The p21-activated kinase (PAK) family comprises six sterile-20 group serine/threonine kinases. In contrast, the type II PAKs bind the Rho-family small GTPases CDC42, RAC1 and RhoV, but are not directly activated by this interaction. The type II PAKs are important for signaling cascades that regulate cell survival, neurite outgrowth and formation of filipodia. We discovered that PAK6 is inhibited by its pseudosubstrate sequence.

The small molecule PF-3758309 was designed as a PAK4-specific inhibitor, but displays in vitro activity against each of the type II PAKs and also PAK1. Though effective in mouse models of cancer, it failed in human clinical trials. We go on to determine crystal structures of PAK6 kinase domain in complex with two ATP-competitive small molecule inhibitors, PF-3758309 and sunitinib. We obtained crystals of PAK6 kinase domain in complex with either PF-3758309 or sunitinib by co-crystallization. These co-crystals diffracted X-rays to Bragg spacings of 1.40 Å and 1.95 Å respectively for the PF-3758309 and sunitinib co-crystals. Good electron density is observed throughout the structures and the conformations of the small molecules are clearly observed. Both co-crystals were obtained in the same crystal form with the activation loop in the extended conformation and residue S560 phosphorylated. Kinases are often classified by the conformation of three residues at the amino-terminus of the activation loop, Asp-Phe-Gly, and we observe that the DFG flip status for both PAK6 crystal structures is ‘DFG-in’. The ATP-binding site is located between the lobes and is occupied by the small molecule inhibitors. M481 is observed in two conformations, which are both shown. Finally, we determined two co-crystal structures of PAK6 in complex with ATP-competitive small molecule inhibitors. These co-crystal structures will facilitate an improved understanding of the modes of targeted inhibition for type II PAKs, and may aid future studies that aim to design inhibitors specific to each of the type II PAK family members.

> GSVTHEQFKAALRMVVDQGDPRLLLDSYVKIGEGSTGIVCLAREKHSGRQVAVKMMDLRKQQRRELLFNEVVIMRDYQHFNVVEMYKSYLVGEELWVLMEFLQGGALTDIVSQVRLNEEQIATVCEAVLQALAYLHAQGVIHRDIKSDSILLTLDGRVKLSDFGFCAQISKDVPKRKSLVGTPYWMAPEVISRSLYATEVDIWSLGIMVIEMVDGEPPYFSDSPVQAMKRLRDSPPPKLKNSHKVSPVLRDFLERMLVRDPQERATAQELLDHPFLLQTGLPECLVPLIQLY>[4x]MSLSKLGYIPNQAARTLITNKTLTIGLIQKSSAPEIRQNPFNSDVLNGINQACNVRGYSTRMTVSENSGDLYHEVKTMIQSKSVDGFILLYSLKDDPIEHLLNEFKVPYLIVGKSLNYENIIHIDNDNIDAAYQLTQYLYHLGHRHILFLQESGHYAV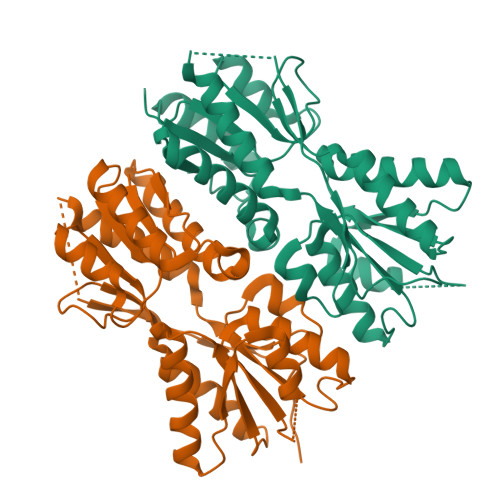TEDRSVGFKQYCDDVKISNDCVVIKSMNDLRDFIKQYCIDASHMPSVIITSDVMLNMQLLNVLYEYQLRIPEDIQTATFNTSFLTENATPSQTSVNINPDVLGFTAGNTIIDVLRNETISFREKLISTQIVERVSTTKIEGHHHHHH>MQYAKISGTGSYLPANRVSNDDLAQKVDTSDEWITARTGIKFRHIAAENEKTSDLAAEAARRALDAAGLDSGEIDLIIVATATPDMQFPSTATIVQQKLGITNGCPAFDVQAVCAGFMYALTTANAYIKSGMAKNALVIGAETFSRIVDWNDRTTCVLFGDGAGAVVLSAADKPGIIHSKLKADGNYLKLLNVPGQIACGKVSGSPYISMDGPGVFKFAVKMLSKIADDVIEEAGYTAAQIDWIVPHQANRRIIESTAKHLGLSMDKVVLTVQDHGNTSAA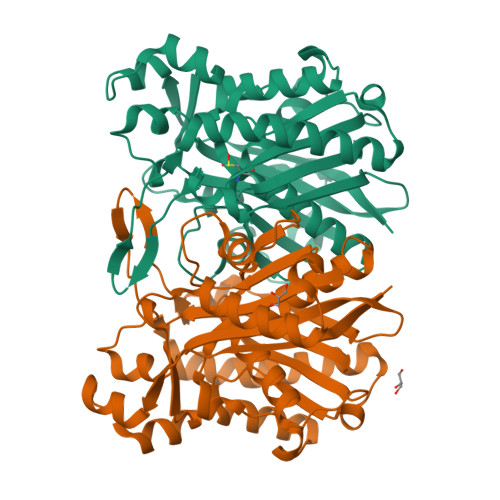SIPLALDTGIRSGQIKRGQNLLLEGIGGGFAWGAVLLQY[2x]>MEIKRRTQEERSAATREALITGARKLWGLRGYAEVGTPEIATEAGVTRGAMYHQFADKAALFRDVVEVVEQDVMARMATLVAASGAATPADAIRAAVDAWLEVSGDPEVRQLILLDAPVVLGWAGFRDVAQRYSLGMTEQLITEAIRAGQLARQPVRPLAQVLIGALDEAAMFIATADDPKRARRETRQVLRRLIDGMLNGKLAAALEHHHHHH[4x]

Here, we show cytokinins induced the strong expression of the M. tuberculosis gene Rv0077c. We found that Rv0077c expression is repressed by a TetR-like transcriptional repressor, Rv0078. As previously reported, Rv0078 forms dimers resembling other TetR-like proteins. Rv0078 has an N-terminal DNA-binding domain (DBD) and a C-terminal ligand-binding domain (LBD).

To gain an understanding of how Rv0078 represses gene expression, we solved the crystal structure of Rv0078 to 1.85 Å by a single-wavelength anomalous dispersion method. The ligand-binding pocket of Rv0078 is largely hydrophobic. Within this pocket, we observed an elongated density resembling a long aliphatic chain of a fatty acid. Gas chromatography-mass spectrometry (GC-MS) of the compounds extracted from Rv0078 purified from Escherichia coli revealed fatty acids commonly found in this organism, and a palmitate molecule fit well with the electron density. A fatty acid carboxylate formed a hydrogen bond with Rv0078 Glu-70, and the long alkyl chain had numerous hydrophobic interactions within the extended ligand pocket. When we purified Rv0078 under denaturing conditions and refolded the protein to remove the lipid, we observed the same EMSA results as we observed with protein purified under native conditions (data not shown), suggesting this fatty acid is unlikely to be the native Rv0078 ligand; however, these data may suggest that the native ligand is fatty acid-like. Interestingly, we found that Trp100 faces the ligand-binding pocket, which suggests Trp100 interacts with the natural ligand. This hypothesis is supported by our data showing an Rv0078W100R mutant was unable to complement the Rv0078 deletion mutant strain (lane 8).> MFKDYTREKFAKENFPDLSKHNNVMASQLTYELYEKYWDKVTPNGVTFDKCIQTGVDNPGNKFYGKKTGCVFGDEYSYECYKEFFDKCIEEIHHFKPSDKHPAPDLDHNKLVGGVFEDKYVKSCRIRCGRSVKGVCLPPAMSRAERRLVEKVVSDALGGLKGDLAGKYYPLTTMNEKDQEQLIEDHFLFEKPTGALLTTSGCARDWPDGRGIWHNNEKNFLVWINEEDHIRVISMQKGGDLKAVFSRFARGLLEVERLMKECGHGLMHNDRLGYICTCPTNMGTVVRASVHLRLAFLEKHPRFDEMLGKLRLGKRGTGGESSLATDSTYDISNWA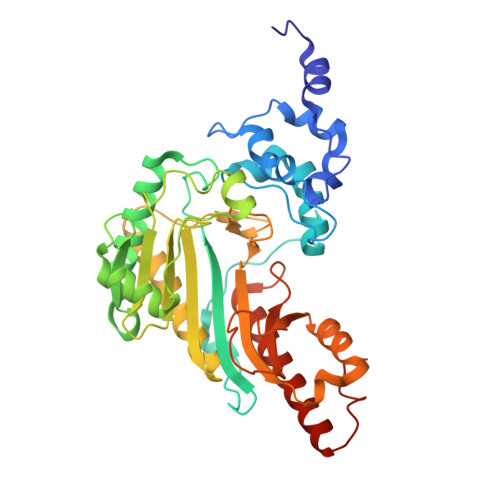RLGKSERELVQVLVDGVNLLIACDKKLEAGQSIDDMIPK>MAAPSPTTTAAAAAAATTHHRVLLPSARPRAAPSSLRLPLRAQPHAHAHAQRARLAAPVAAAAPAPAASTASPESPASGAVAGKPTVLVAEKLGAAGLALLREFANVDCSYGLSPEDLRAKISLCDALIVRSGTKVGRDVFEASGGRLRVVGRAGVGIDNVDLAAATEHGCLVVNAPTANTVAAAEHGIALLTAMARNIAQADASLKAGKWQRNKYVGVSLVGKTLAILGFGKVGSEVARRAKGLGMHVIAHDPYASADRARAIGVELVSMEEAMTTADFILLHMPLTPATDKMLNDEAFAKMKKGVRIINVARGGVIDEEALVRALDSGV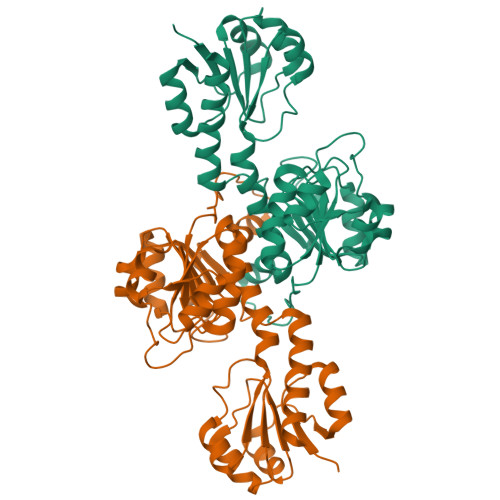VAQAALDVFTKEPPAADNKLVLHGNVTVTPHLGASTVEAQEGVAIEIAEAVIGALK[2x]> MSNISRQAYADMFGPTVGDKVRLADTELWIEVEDDLTTYGEEVKFGGGKVIRDGMGQGQMLAADCVDLVL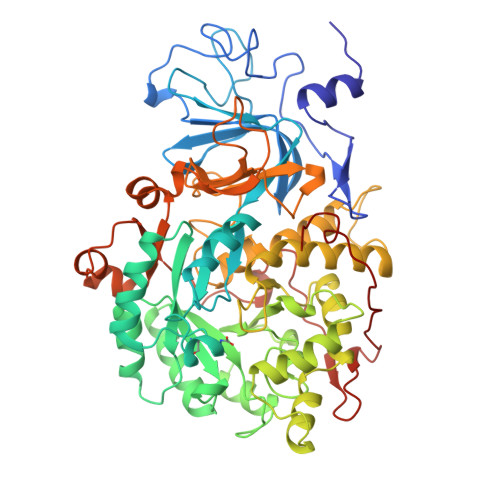TNALIVDHWGIVKADIGVKDGRIFAIGKAGNPDIQPNVTIPIGAATEVIAAEGKIVTAGGIDTHIHWICPQQAEEALVSGVTTMVGGGTGPAAGTHATTCTPGPWYISRMLQAADSLPVNIGLLGKGNVSQPDALREQVAAGVIGLKIHEDWGATPAAIDCALTVADEMDIQVALHSDTLNESGFVEDTLAAIGGRTIHTFHTEGAGGGHAPDIITACAHPNILPSSTNPTLPYTLNTIDEHLDMLMVYHHLDPDIAEDVAFAESRIRRETIAAEDVLHDLGAFSLTSSDSQAMGRVGEVILRTWQVAHRMKVQRGALAEETGDNDNFRVKRYIAKYTINPALTHGIAHEVGSIEVGKLADLVVWSPAFFGVKPATVIKGGMIAIAPMGDINASIPTPQPVHYRPMFGALGSARHHCRLTFLSQAAAANGVAERLNLRSAIAVVKGCRTVQKADMVHNSLQPNITVDAQTYEVRVDGELITSEPADVLPMAQRYFLF> MGSSHHHHHHSQDPENLYFQGSDQHDERRRFHRIAFDA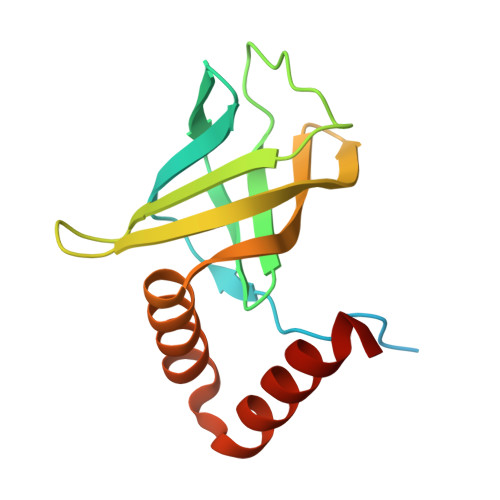DSEILQGERRWEVLLHDVSLHGILVGQPQDWNGDPQRPFEARLYLGLDVLIRMEISLAWARDGLLGFECQHIDLDSISHLRRLVELNLGDEELLERELALLVSAHDD>[6x]GSGQMFGNGKGSYFI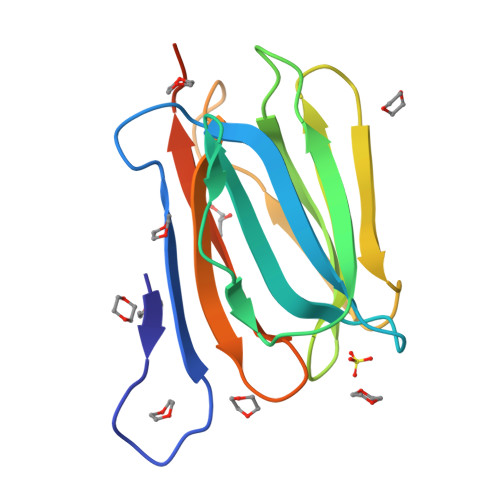TSKDNETGITGIRVFVGPVGLIKSIQVRYGSSWSEKYGIPGGKAHELILHPGEHIISIYGRYRTFLQHVTLITNQGRSASFGLETGKGFFAAPNLTGQVLEGVYGQFWLYGITGIGFTWGFPREGLASVLPSDDPF> AMTYHLDVVSAEQQMFSGLVEKIQVT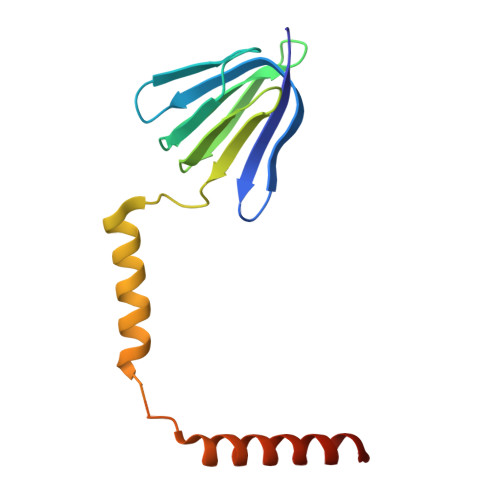GSEGELGIYPGHAPLLTAIKPGMIRIVKQHGHEEFIYLSGGILEVQPGNVTVLADTAIRGQDLDEARAMEAKRKAEEHISSSHGDVDYAQASAELAKAIAQLRVIELTKKAM>QEVEFDIPPQALGSALQEFGRQADIQVLYRPEEVRNKRSSAIKGKLEPNQAITELLRGTGASVDFQGNAITISVAEAADSSVDLGATMITSNQLGTITEDSGSYTPGTIATATRLVLTPRETPQSITVVTRQNMDDFGLNNIDDVMRHTPGITVSAYDTDRNNYYARGFSINNFQYDGIPSTARNVGYSAGNTLSDMAIYDRVEVLKGATGLLTGAGSLGATINLIRKKPTHEFKGHVELGAGSWDNYRSELDVSGPLTESGNVRGRAVAAYQDKHSFMDHYERKTSVYYGILEFDLNPDTMLTVGADYQDNDPKGSGWSGSFPLFDSQGNRNDVSRSFNNGAKWSSWEQYTRTVFANLEHNFANGWVGKVQLDHKINGYHAPLGAIMGDWPAPDNSAKIVAQKYTGETKSNSLDIYLTGPFQFLGREHELVVGTSASFSHWEGKSYWNLRNYDNTTDDFINWDGDIGKPDWGTPSQYIDDKTRQLGSYMTARFNVTDDLNLFLGGRVVDYRVTGLNPTIRESGRFIPYVGAVYDLNDTYS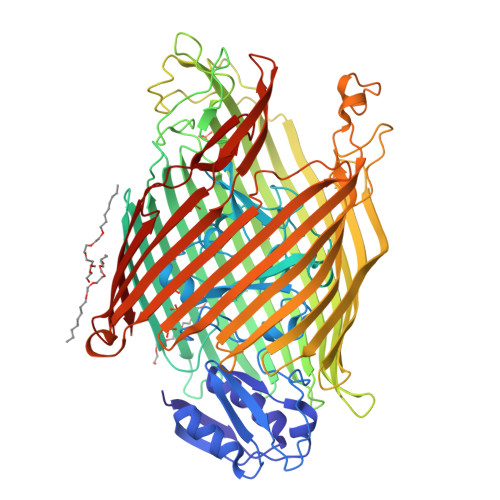VYASYTDIFMPQDSWYRDSSNKLLEPDEGQNYEIGIKGEYLDGRLNTSLAYFEIHEENRAEEDALYNSKPTNPAITYAYKGIKAKTKGYEAEISGELAPGWQVQAGYTHKIIRDDSGKKVSTWEPQDQLSLYTSYKFKGALDKLTVGGGARWQGKSWQMVYNNPRSRWEKFSQEDYWLVDLMARYQITDKLSASVNVNNVFDKTYYTNIGFYTSASYGDPRNLMFSTRWDF[2x];> SKGKSSGAKS> GUGGUCUGAUGAGGCC;> GCCGAAACUCGUAAGAGUCACC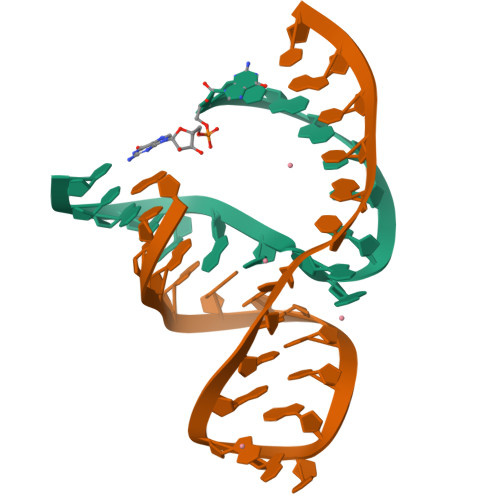AC> MVKLSSDINLRDFGNNEYLSSVQDEAIRFATEQTDEILSLYSQHADTEGGRYVCADTFKELFPAFENKEDRATVNNAIHNSAAVLSSTQFDEVLKRDEPQKKEVIFVTGIPGSGATSTVKNMMMQDTTKLLFEGQLARPQSAFRKIEQCLERNLEVTIVAVSMRAERASDNTYKRFNEYGRGASIGIMADIQANLPDGLKQIRDKFGDAVKIVGINQDRNSEFIDKFDDVIKMLSLGSQEQILGRLAEKIQSDFDSGKISRECFNQAKGSMDLESVFAKKEYSQQRVVTNSKGVTLETKSANELWS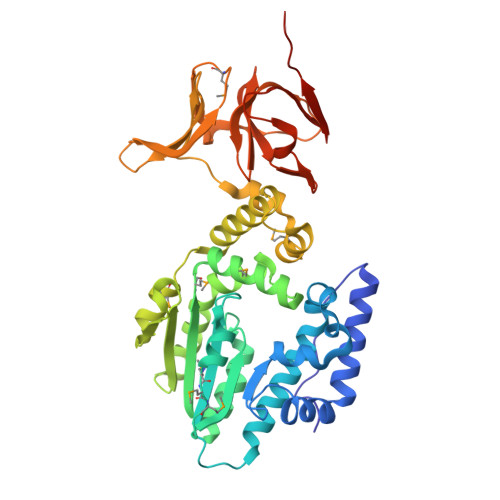KVEQIPVTGMKAGIYLLGQAKKAETGQTYSGEIIYKDAAAVFQKTKNGLVRHNATHNEERLAKLVEIGQNVSIGSNKGKLIVKSLEYSAKKSISR>SAPRPCQAPQQWEGRQVMYQQSSGRNSRALLSYDGLNQRVRVLDERKALIPCKRLFEYILLYKDGVMFQIDQATKQCSKMTLTQPWDPLDIPQNSTFEDQYSIGGPQEQITVQEWSDRKSARSYETWIGIYTVKDCYPVQETFTINYSVILSTRFFDIQLGIKDPSVFTPPSTCQMAQLEKMSEDCSWHHHHHH[2x]

EPDR1 is a member of the ependymin-related (EPDR) family of proteins. The crystal structure confirms that EPDR1 adopts the highly curved β-sheet fold that had been previously observed only in bacterial proteins. Two EPDR1 chains associate into a tight homodimer through extensive hydrophilic contacts between the convex surfaces of shelf-II. At acidic pH, EPDR1 can bind to liposomes that contain the anionic lipid bis-monoacylglycero-phosphate (BMP) or the ganglioside GM1, consistent with a role in the degradation or transport of lipids and/or lipoproteins within the lysosome.

EPDR1 contains a single glycosylation site at residue Asn130 of loop L7 on the back-side of the glove. In the structure of glycosylated EPDR1, the hydrophobic grooves from the two monomers each contain a long continuous tube of electron density, which can be due to a copurifying lipid or a PEG molecule contributed from the crystallization solution. We were not able to identify copurifying lipids by mass spectroscopy. We modeled this ligand as an extended PEG chain; the U-shaped path of the unidentified ligand follows the floor of the groove and was similar in both protomers. The buried ligand is in van der Waals contact with the hydrophobic side chains of residues M54, L67, Y69, V76, V78, Y94, L96, Y98, M103 on shelf-I, F179, I181, I186, L187, F191 on shelf-II and W122 and L125 in L7. The rim of the groove is rich in charged and polar residues and there is a notable clustering of the conserved, exposed polar side chains D123, K155 and E161 at one end of the groove. Structures of EPDR1 with and without an unexpected bound ligand, likely to be a PEG molecule from the crystallization condition, identify an elongated, surface-exposed hydrophobic binding groove in each chain of the homodimer. All three of the crystallographically independent EPDR1 homodimers (one dimer from crystals of the glycosylated protein, and two dimers from crystals of the deglycosylated protein) are similar to each other with Cα RSMDs less than 0.6 Å, indicating little variability within the chains and across the homodimer interface. EPDR1 has two non-overlapping lipid-binding grooves on the same flat surface of the homodimer, and we presume that this allows the half dome-shaped protein to bind to membranes with an extensive contact surface for the binding and possible extraction and solubilization of target lipids.> M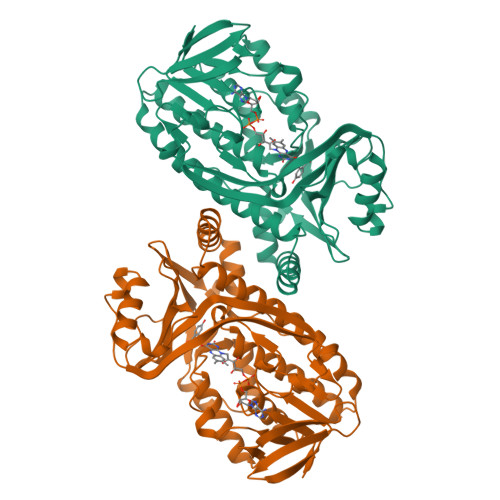KTQVAIIGAGPSGLLLGQLLHKAGIDNVILERQTPDYVLGRIRAGVLEQGMVDLLREAGVDRRMARDGLVHEGVEIAFAGQRRRIDLKRLSGGKTVTVYGQTEVTRDLMEAREASGATTVYQAAEVRLHDLQGERPYVTFERDGERLRLDCDYIAGCDGFHGISRQSIPAERLKVFERVYPFGWLGLLADTPPVSHELIYANHPRGFALCSQRSATRSRYYVQVPLTEKVEDWSDERFWTELKARLPAEVAEKLVTGPSLEKSIAPLRSFVVEPMQHGRLFLAGDAAHIVPPTGAKGLNLAASDVSTLYRLLLKAYREGRGELLERYSAICLRRIWKAERFSWWMTSVLHRFPDTDAFSQRIQQTELEYYLGSEAGLATIAENYVGLPYEEIE> GMDISGRDVETRLTLAREFMSGVDELPTVPDIVLRIAGKLNDPDVAIDEVADLLLQDQVLTARVVHLANSPLYSAARPISSIRDAVIYLGLDLLREAIFTCAIVDLFKTGKGPLNRSTLWAHSLGVARIAKLIAERTGFLNPVNVYVAGLLHDVGEVFINFFRGKEFSQVVTLVDEEKITFGQAEERLFGTSHCEVGFALAKRWSLNEFICDTILYHHDIEAVPYKQAAIVAMVAFADEYCT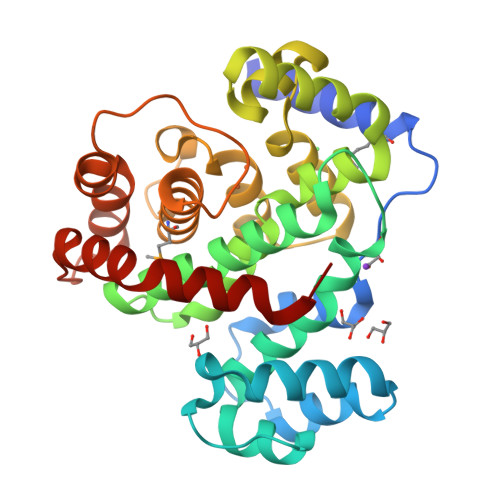LRRLGFEGHKPVDSVRTLLENHPSWGVIRRSLGGSDFDEKLIVAELDSSIVEIRAAVDELFLL>SGAYWMSPTADDIRAMNRMQRQRVVGFTVGRENV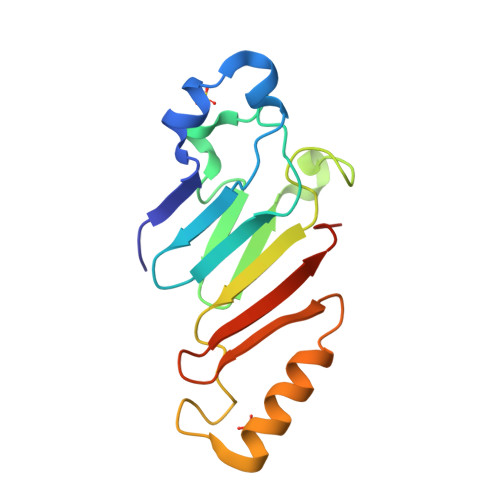GSVQFKVPVDLSNINLDDLFGTIVILEPRSATVYPNAAKKPPMGKGLNVPALISLEHSWPRGGPTIKGRRLERHIERLKSIPDTTFESYDPETGVWAFSVEHFATYGLGD[2x]> FQKIYSPTQLANAMKLVRQQNGWT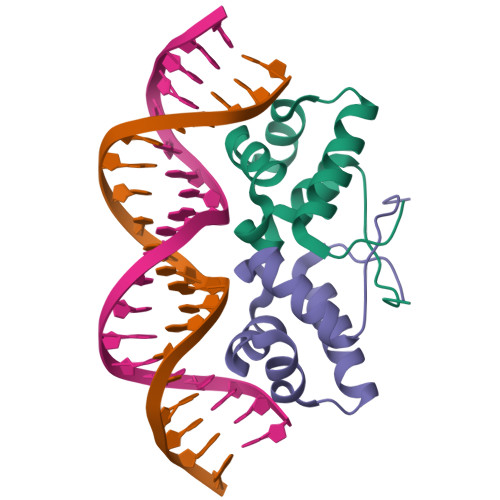QSELAKKIGIKQATISNFENNPDNTTLTTFFKILQSLELSMTLCDAK methyl 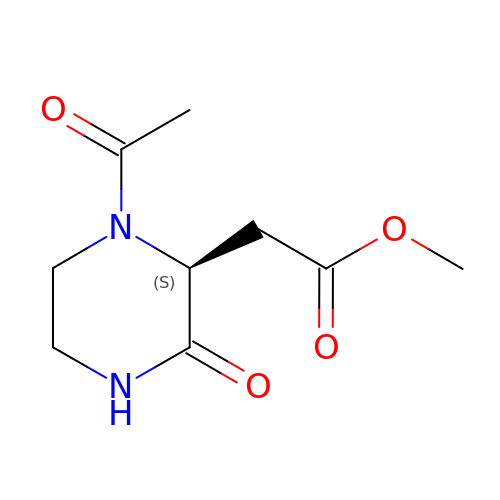2-[(2~{S})-1-ethanoyl-3-oxidanylidene-piperazin-2-yl]ethanoate | C9 H14 N2 O4 | XXDJRDKSNTXOKT-ZETCQYMHSA-N> GAMDISPTNHHEMLQNLQTVVNELYREDVDY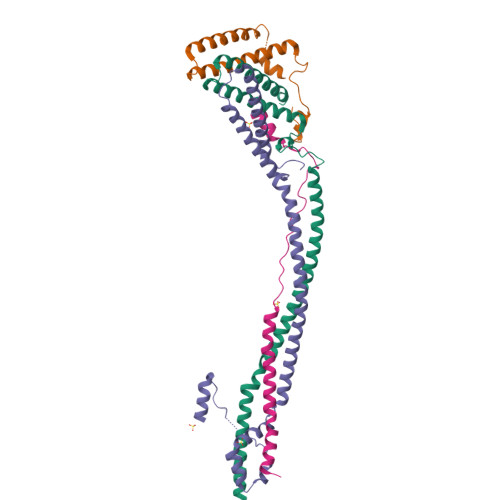VADKILTRQTVMQESIARFHEIIAIDKNHLRAVEQAIEQTMHSLNAQIDVLTANRAKVQQFSSTSHVDDEDVNSIAVAKTDGLNQLYNLVAQDYALTDTIECLSRMLHRGTIPLDTFVKQGRELARQQFLVRWHIQRITSPLS;> MQKHNIKLNQNQDISQLFHDEVPLFDNSITSKDKEVIETLSEIYSIVITLDHVEKAYLKDSIDDTQYTNTVDKLLKQFKVYLNSQNKEEINKHFQSIEAFADTYNITASNAITRLERG;> SRLDIIRAEMDVVPSPGLPEKVNEKSKNIPLPEGINLLSSKEIIDLIQTHRHQLELYVTKFNPLTDFAGKIHAFRDQFKQLEENFEDLHEQKDKVQALLENARILESKYVASWQDYHSEFSKKYGDIALKKKLEQNTKKLDEESSQLETTTRSIDSADDLDQFIKNYLDIRTQYHLRREKLATWDKQGNLKY;> MNVEELLRRIPLYNKYGKDFPQETVTRFQMPEFKLPALQPTRDLLCPWYEECDNITKVCQLHDSSNKKFDQWYKEQYLS>[4x]MGHHHHHHMSKLLSGQVALVTGGAAGIGRATAQAFAAAGVKVVVADLDSAGGEGTVEAIRQAGGEAVFIRCDVTRDAEVKALVEGCAAAYGRLDYAFNNAGIEIEQGKLADGNEAEFDAIMAVNVKGVWLCMKHQIPLMLAQGGGAIVNTASVAGLGAAPKMSIYAASKHAVIGLTKSAAIEYAKKGIRVNAVCPAVIDTDMFRRAYEADPRKAEFAAAMHPLGRVGRVEEIAAAVLYLCSDNAGF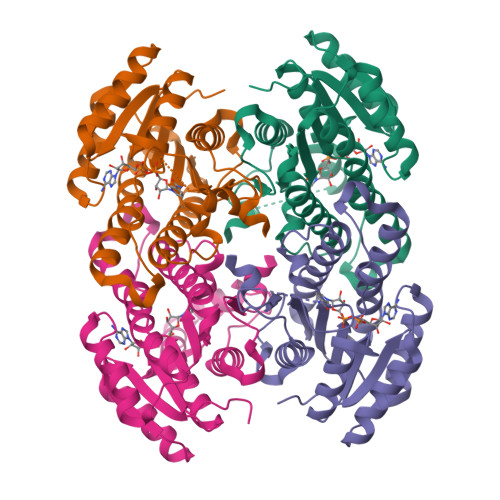TTGIALPVDGGATAI>[2x]MGMLEARELLCERDERTLFSGLSFTLNAGEWVQITGSNGAGKTTLLRLLTGLSRPDAGEVLWQGQPLHQVRDSYHQNLLWIGHQPGIKTRLTALENLHFYHRDGDTAQCLEALAQAGLAGFEDIPVNQLSAGQQRRVALARLWLTRATLWILDEPFTAIDVNGVDRLTQRMAQHTEQGGIVILTTHQPLNVAESKIRRISLT;>MMFWRIFRLELRVAFRHSAEIANPLWFFLIVITLFPLSIGPEPQLLARIAPGIIWVAALLSSLLALERLFRDDLQDGSLEQLMLLPLPLPAVVLAKVMAHWMVTGLPLLILSPLVAMLLGMDVYGWQVMALTLLLGTPTLGFLGAPGVALTVGLKRGGVLLSILVLPLTIPLLIFATAAMDAASMHLPVDGYLAILGALLAGTATLSPFATAAALRISIQ[2x];> MWKTLHQLAIPPRLYQICGWFIPWLAIASVVVLTVGWIWGFGFAPADYQQGNSYRIIYLHVPAAIWSMGIYASMAVAAFIGLVWQMKMANLAVAAMAPIGAVFTFIALVTGSAWGKPMWGTWWVWDARLTSELVLLFLYVGVIALWHAFDDRRLAGRAAGILVLIGVVNLPIIHYSVEWWNTLHQGSTRMQQSIDPAMRSPLRWSIFGFLLLSATLTLMRMRNLILLMEKRRPWVSELILKRGRK;> MTPAFASWNEFFAMGGYAFFVWLAVVMTVIPLVVLVVHSVMQHRAILRGVAQQRAREARLRAAQQQEAA

The cytochrome c maturation system I, consisting of eight membrane proteins (CcmABCDEFGH), results in the attachment of heme to cysteine residues of cytochrome c proteins. CcmABCD represents an ABC transporter complex using the energy of ATP hydrolysis for the transfer of heme from one binding partner (CcmC) to another (CcmE). Our cryo-EM structures reveal that CcmA2B2 form a homodimer which is an ABC transporter analog. CcmC which harbors the heme-binding site is attached to two CcmBs with two coupling helices TM4 and TM5 on CcmC, respectively.

A conformation with only one ATP bound, near CcmC, exhibits a “semi-open” inward-facing conformation. In this semi-open state, heme is loosely associated in the CcmC binding site and does not form a coordination bond with P-His1. In a second conformation with heme, in a semi-open NBD state, P-His1 is not an axial ligand, for the distance between heme iron and P-His1 is 4.4 Å and the angle between the line of P-His1 N(δ)–heme iron and the heme plane is ~50°. In both conformations with heme, P-His2 is not a ligand and the entire P-His2 loop is located near the CcmC:B interface. CcmC has a hydrophobic tryptophan-rich motif (WWD domain) of which at least two tryptophan residues W114C and W119C are in close contact with the heme in both heme-bound conformations. The semi-open NBD state shows a similar but smaller conformational change as the open NBD state. We propose that we have trapped heme in conformations whereby the CcmABCD cycle of ATP hydrolysis weakens interactions with heme leading towards release.>[10x]MIIVTGGAGFIGSNI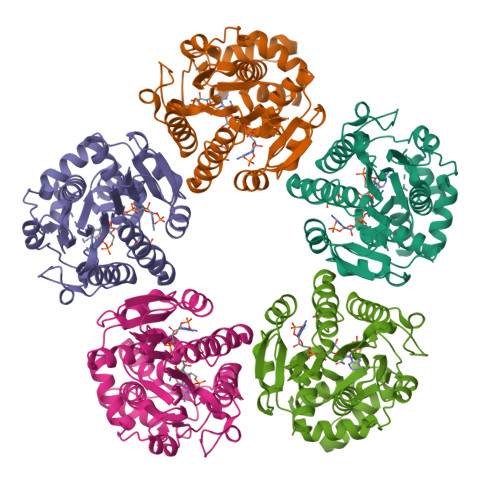VKALNDKGITDILVVDNLKDGTKFVNLVDLNIADYMDKEDFLIQIMAGEEFGDVEAIFHEGACSSTTEWDGKYMMDNNYQYSKELLHYCLEREIPFLYASSAATYGGRTSDFIESREYEKPLNVYGYSKFLFDEYVRQILPEANSQIVGFRYFNVYGPREGHKGSMASVAFHLNTQLNNGESPKLFEGSENFKRDFVYVGDVADVNLWFLENGVSGIFNLGTGRAESFQAVADATLAYHKKGQIEYIPFPDKLKGRYQAFTQADLTNLRAAGYDKPFKTVAEGVTEYMAWLNRDA> KRVKIAKPDLSSFQPGSIIKIRLQDFVTYTLTEFNLSPSLNMIIGPNGSGKSTFVCAVCLGLAGKPEYIGRSKKVEDFIKNGQDVSKIEITLKNSPNVTDIEYIDARDETIKITRIITRSKRRSDYLINDYQVSESVVKTLVAQLNIQLDNLCQFLSQERVEEFARLKSVKLLVETIRSIDASLLDVLDELRELQGNEQSLQKDLDFKKAKIVHLRQESDKLRKSVESLRDFQNKKGEIELHSQLLPYVKVKDHKEKLNIYKEEYERAKANLRAILKDKKPFANTKKTLENQVEELTEKCSLKTDEFLKAKEKINEIFEKLNTIRDEVIKKKNQNEYYRGRTKKLQATIISTKEDFLRSQEILAQTHLPEKSVFEDIDIKRKEIINKEGEIRDLISEIDAKANAINHEMRSIQRQAESKTKSLTTTDKIGILNQDQDLKEVRDAVLMVREHPEMKDKILEPPIMTVSAINAQFAAYLAQCVDYNTSKALTVVDSDSYKLFANPILDKFKVNLRELSSADTTPPVPAETVRDLGFEGYLSDFITGDKRVMKMLCQTSKIHTIPVSRRELTPAQIKKLITPRPNGKILFKRIIHGNRLVDIKQSAYGSKQVFPTDVSIKQTNFYQGSIMSNEQKIRIENEIINLKNEYNDRKSTLDALSNQKSGYRHELSELASKNDDINREAHQLNEIRKKYTMRKSTIETLREKLDQLKREAR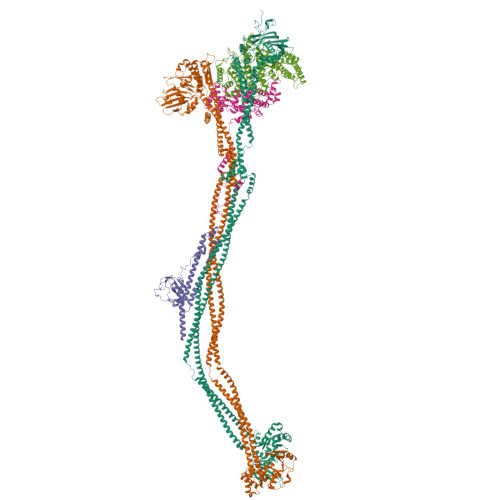KDVSQKIKDIDDQIQQLLLKQRHLLSKMASSMKSLKNCQKELISTQILQFEAQNMDVSMNDVIGFFNEREADLKSQYEDKKKFVKEARDTPEFQSWMREIRSYDQDTKEKLNKVAEKYEEEGNFNLSFVQDVLDKLESEIAMVNHDESAVTILDQVTAELRELEHTVPQQSKDLETIKAKLKEDHAVLEPKLDDIVSKISARFARLFNNVGSAGAVRLEKPKDYAEWKIEIMVKFRDNAPLKKLDSHTQSGGERAVSTVLYMIALQEFTSAPFRVVDEINQGMDSRNERIVHKAMVENACAENTSQYFLITPKLLTGLHYHEKMRIHCVMAGSWIPNPSEDPKMIHFGETSNYSFD;> MISTTISGKRPIEQVDDELLSLTAQQENEEQQQQRKRRRHQFAPMTQFNSNTLDEDSGFRSSSDVATADQDNFLEESPSGYIKKVILRNFMCHEHFELELGSRLNFIVGNNGSGKSAILTAITIGLGAKASETNRGSSLKDLIREGCYSAKIILHLDNSKYGAYQQGIFGNEIIVERIIKRDGPASFSLRSENGKEISNKKKDIQTVVDYFSVPVSNPMCFLSQDAARSFLTASTSQDKYSHFMKGTLLQEITENLLYASAIHDSAQENMALHLENLKSLKAEYEDAKKLLRELNQTSDLNERKMLLQAKSLWIDVAHNTDACKNLENEISGIQQKVDEVTEKIRNRQEKIERYTSDGTTIEAQIDAKVIYVNEKDSEHQNARELLRDVKSRFEKEKSNQAEAQSNIDQGRKKVDALNKTIAHLEEELTKEMGGDKDQMRQELEQLEKANEKLREVNNSLVVSAQDVKNEERDIQHERESELRTISRSIQNKKVELQNIAKGNDTFLMNFDRNMDRLLRTIEQRKNEFETPAIGPLGSLVTIRKGFEKWTRSIQRAISSSLNAFVVSNPKDNRLFRDIMRSCGIRSNIPIVTYCLSQFDYSKGRAHGNYPTIVDALEFSKPEIECLFVDLSRIERIVLIEDKNEARNFLQRNPVNVNMALSLRDRRSGFQLSGGYRLDTVTYQDKIRLKVNSSSDNGTQYLKDLIEQETKELQNIRDRYEEKLSEVRSRLKEIDGRLKSTKNEMRKTNFRMTELKMNVGKVVDTGILNSKINERKNQEQAIASYEAAKEELGLKIEQIAQEAQPIKEQYDSTKLALVEAQDELQQLKEDINSRQSKIQKYKDDTIYYEDKKKVYLENIKKIEVNVAALKEGIQRQIQNACAFCSKERIENVDLPDTQEEIKRELDKVSRMIQKAEKSLGLSQEEVIALFEKCRNKYKEGQKKYMEIDEALNRLHNSLKARDQNYKNAEKGTCFDADMDFRASLKVRKFSGNLSFIKDTKSLEIYILTTNDEKARNVDTLSGGEKSFSQMALLLATWKPMRSRIIALDEFDVFMDQVNRKIGTTLIVKKLKDIARTQTIIITPQDIGKIADIDSSGVSIHRMRDP;> MALNDNPIPKSVPLHPKSGKYFHNLHARDLSNIYQQCYKQIDETINQLVDSTSPSTIGIEEQVADITSTYKLLSTYESESNSFDEHIKDLKKNFKQSSDACPQIDLSTWDKYRTGELTAPKLSELYLNMPTPEPATMVNNTDTLKILKVLPYIWNDPTCVIPDLQNPADEDDLQIEGGKIELTCPITCKPYEAPLISRKCNHVFDRDGIQNYLQGYTTRDCPQAACSQVVSMRDFVRDPIMELRCKIAKMKESQEQDKRSSQAIDVL;> PILKRTIISKRKAPSNNEDEEIVKTPRKLVNYVPLKIFNLGDSFDDTITTTVAKLQDLKKEILDSPRSNKSIVITSNTVAKSELQKSIKFSGSIPEIYLDVVTKETISDKYKDWHFISKNCHYEQLMDLEMKDTAYSFLFGSSRSQGKVPEFVHLKCPSITNLLVLFGVNQEKCNSLKINYEKKENSRYDNLCTIFPVNKMLKFLMYFYSDDDNDDVREFFLKAFICLILDRKVFNAMESDHRLCFKVLELFNEAHFINSYFEIVDKNDFFLHYRLLQIFPHLQSALLRRRFSEKQGRTETIQQNIIKEFNEFFDCKNYKNLLYFILTMYGSKFIPFGPKCQVTEYFKDCILDISNETTNDVEISILKGILNLFSKIR;> MDGALINSVLYVSPRNGAHYFVELTEKHLLAFEMLNSMCLLENYDHVLLFLECQFGKSHNLAVIPFDIILVLFTLSTLSEYYKEPILRANDPYNTSRETLSRRALKLLQKYLAILKEFDSEQYNLYDLELLRCQFFLAIDTLTPKKQKWGFDRFRRTKSESGVTYRQNASVDPELDQAKTFKNPYRSYISCLEQRNTILGNRLLNLKLNEPGEFINMILWTLSNSLQESTPLFLSSHEIWMPLLEILIDLFSCRQDYFIQHEVAQNVSKSLFVQRLSESPLAVFFESLNTRNFANRFSEYVFLNCDYKLPSDNYATPVHPVYNGENTIVDTYIPTIKCSPLYKSQKSLALRRKLIGSCFKLLLRVPDGHRLITPRIVADDVIQGISRTLASFNDILQFKKFFMTENLSQESYFIPLLAEGTLSEILKDTQECVVILTLVENLSDGVSFCNEVIGLVKSKCFAFTEQCSQASYEEAVLNIEKCDVCLLVLLRYLLHLIGTEAILDAKEQLEMLHAIEKNDSGRRQWAKALNLGNDPPLLYPIVSQMFGVHDKSVIIE The biocatalytic reduction of the oxime moiety to the corresponding amine group has only recently been found to be a promiscuous activity of ene-reductases transforming α-oximo β-keto esters. By studying the crystal structures of enzyme oxime complexes, analyzing molecular dynamics simulations, and investigating biocatalytic cascades and possible intermediates, we obtained evidence that the reaction proceeds via an imine intermediate and not via the hydroxylamine intermediate. To gain more insight into the reaction pathway, we determined the crystal structures of the two enzymes OPR3 and XenA in complex with the oxime substrates 1a–c, either by co-crystallization or by soaking. All the crystal structures obtained had a high resolution (1.9–1.35 Å) and showed clear electron density features for the oximes.

To assess if the introduced amino acid exchanges affected the overall structure and the binding of the oxime, we also crystallized the tyrosine variants in complex with selected oxime substrates. The protomers in the crystal structures of the tyrosine variants are perfectly superimposable with the ones of the wild-type enzymes, confirming that the exchanges did not lead to major structural alterations. The only exception was found for XenA Y183F in complex with oxime 1b: while the electron density of the substrate was clear in the wild-type enzyme—and only the productive binding mode could be modeled in it—the density for the oxime appears less defined in the Y183F variant, and both the productive and the non-productive binding mode could be fit in the density. Binding pose metadynamics performed on both productive and non-productive binding modes (non-productive modeled from the crystal structure of XenA_Y183F, vide infra) showed that the productive binding mode appeared to have higher stability than the non-productive binding mode. In fact, it presents a lower root-mean-square deviation (RMSD) than the non-productive binding pose, which shows a steep RMSD increase over time, indicating poor binding of the substrate in the active site. Tyrosine 183, the canonical proton donor of XenA,55 is also found at a hydrogen bond distance from the Cα of the oxime. Hydride transfer to the oxime nitrogen followed by proton transfer from the canonical tyrosine would lead to the formation of the hydroxylamine (pathway B). The calculated high Kd for oxime 1b clearly indicates this enzyme’s low affinity for the substrate and might explain why this enzyme performed poorly in the biotransformation of the other oximes in our previous work. Both the Y183F and the Y27F variants of XenA showed a non-Michaelis–Menten behavior, with a linear increase of the rate over the concentration (bottom right).

>[2x]MSALFEPYTLKDVTLRNRIAIPPMCQYMAEDGLINDWHQVHYASMARGGAGLLVVEATAVAPEGRITPGCAGIWSDAHAQAFVPVVQAIKAAGSVPGIQIAHAGRKASANRPWEGDDHIGADDARGWETIAPSAIAFGAHLPNVPRAMTLDDIARVKQDFVDAARRARDAGFEWIELHFAHGFLGQSFFSEHSNKRTDAYGGSFDNRSRFLLETLAAVREVWPENLPLTARFGVLEYDGRDEQTLEESIELARRFKAGGLDLLSVSVGFTIPETNIPWGPAFMGPIAERVRREAKLPVTSAWGFGTPQLAEAALQANQLDLVSVGRAHLADPHWAYFAAKELGVEKASWTLPAPYAHWLERYRLEHHHHHH> GSHMMPQLQFKDAFWCRDFTAHTGYEVLLQRLLDGRKMCKDMEELLRQRAQAEERYGKELVQIARKAGGQTEINSLRASFDSLKQQMENVGSSHIQLALTLREE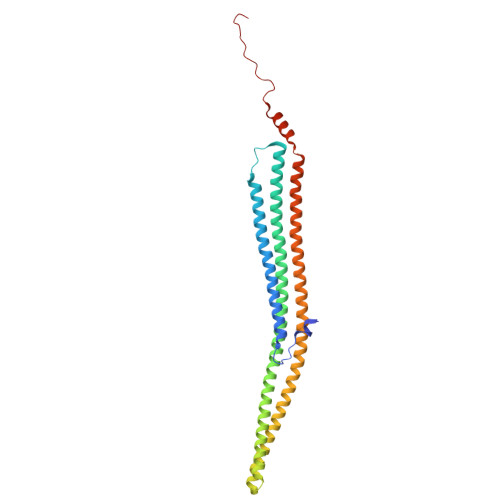LRSLEEFRERQKEQRKKYEAVMDRVQKSKLSLYKKAMESKKTYEQKCRDADDAEQAFERISANGHQKQVEKSQNKARQCKDSATEAERVYRQSIAQLEKVRAEWEQEHRTTCEAFQLQEFDRLTILRNALWVHSNQLSMQCVKDDELYEEVRLTLEGCSIDADIDSFIQAKSTGTEPPAPVPYQNYYD7A-[(4-cyanophenyl)methyl]-6-(3,5-dichlorophenyl)-5-oxo-2,3,5,7A-tetrahydro-1H-pyrrolo[1,2-A]pyrrole-7-carbonitrile | C22 H15 Cl2 N3 O | 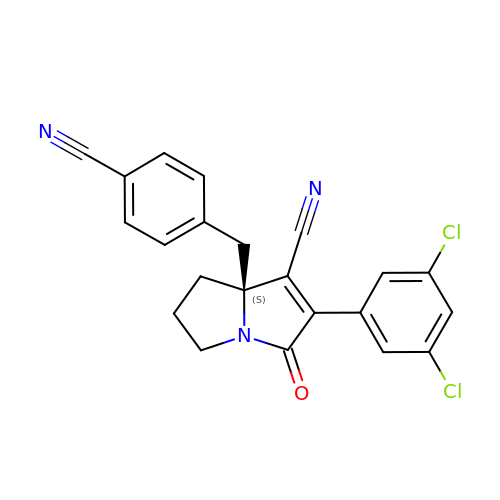TZCXQSNBTXDAJG-QFIPXVFZSA-N> MHHHHHHPPKRAALIQNLRDSYTETSSFAVIEEWAAGTLQEIEGIAKAAAEAHGVIRNSTYGRAQAEKSPEQLLGVLQRYQDLCHNVYCQAETIRTVIAIRIPEHKEEDNLGVA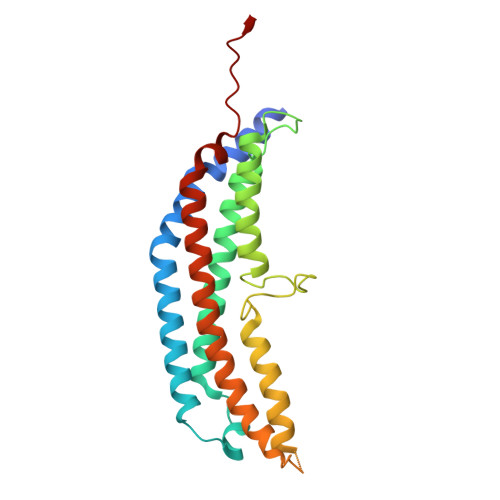VQHAVLKIIDELEIKTLGSGEKSGSGGAPTPIGMYALREYLSARSTVEDKLLGSVDAESGKTKGGSQSPSLLLELRQIDADFMLKVELATTHLSTMVRAVINAYLLNWKKLIQPRTGSDHMVS>[2x]MSFGGKSMSEHSAIVTWKRKDSEAFTDNQYS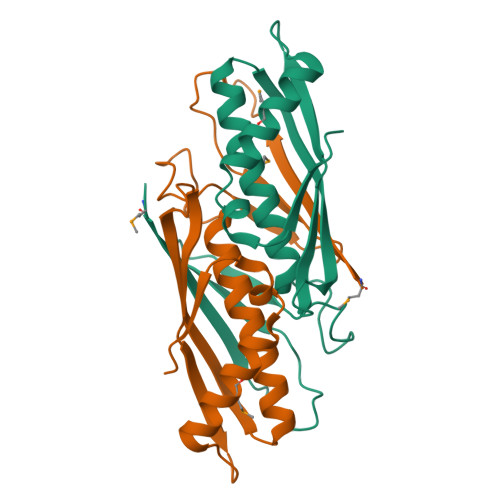RAHTWEFDGGSKILASASPHVVPVPLSVEANVDPEEAFVAALSSCHMLVFLSIAAKQRYLVESYTDNAVGILGKNSKGKTSVTKVVLRPQVVFSGTSKPTLQQLEKMHHLAHENCFIANSVETEVVTEIIA>MRGSHHHHHHTDPTGATFPEEAIADLSVNMYNRLRATGEDENILFSPLSIALAMGMMELGAQGSTQKEIRHSMGYDSLKNGEEFSFLKEFSNMVTAKESQYVMKIANSLFVQNGFHVNEEFLQMMKKYFNAAVNHVDFSQNVAVANYINKWVENNTNNLVKDLVSPRDFDAATYLALINAVYFKGNWKSQFRPENTRTFSFTKDDESEVQIPMMYQQGEFYYGEFSDGSNEAGGIYQVLEIPYEGDEISMMLVLSRQEV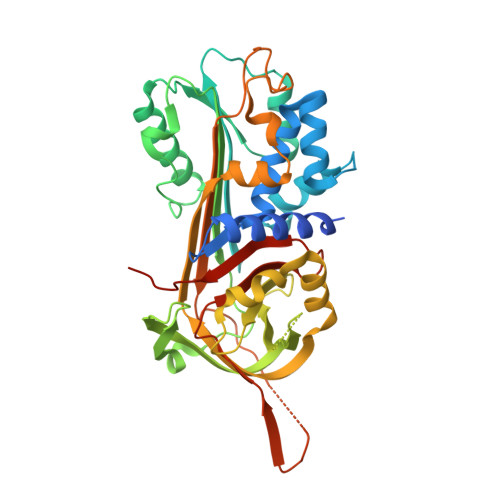PLATLEPLVKAQLVEEWANSVKKQKVEVYLPRFTVEQEIDLKDVLKALGITEIFIKDANLTGLSDNKEIFLSKAIHKSFLEVNEEGSEAAAVSGMIAISRMAVLYPQVIVDHPFFFLIRNRRTGTILFMGRVMHPETMNTSGHDFEEL[5x]> MRGSHHHHHHGSMPETNPNAPPRPDSLLNPSDALKHLEEYPRGDGLSLQE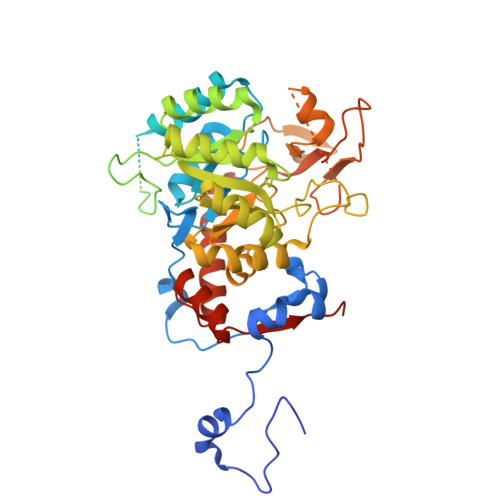LMDSRKNGGLTYNDFLVLPGHINFPASDVSLQSKATKNIVLNTPFLSSPMDTVTEDRMAIALALHGGLGIIHHNCSAEEQAAMVRRVKKYENGFITDPLCLGPDATVGDVLEIKAKFGFCGVPITETGEPDSKLLGIVTGRDVQFQDAETPIKSVMTTEVVTGSSPITLEKANSLLRETKKGKLPIVDSNGHLVSLVARSDLLKNQNYPYASKVPESKQLYCGAAIGTRPGDKDRLKLLAEAGLDVVVLDSSQGNSVYQIEFIKWIKQTYPKIDVIAGNVVTREQAAQLIAAGADGLRIGMGSGSICITQEVMAVGRPQGTAVYAVAEFASRFGIPCIADGGIGNIGHIAKALALGASAVMMGGLLAGTTESPGEYFYHEGKRVKVYRGMGSIEAMEHTQRGSASGKRSILGLDNAATARYFSEADAVKVAQGVSGDVADKGSINKFVPYLFTGLQHSLQDAAIKSVSELHSCARSGSLRFELRTASAQLEGGVHGLNSYTKRLFA> GHMLQNNTDYPFEANNPYMYHENPMEEGLSMLKLANLAEAALAFEAVCQAAPEREEAWRSLGLTQAENEKDGLAIIALNHARMLDPKDIAVHAALAVSHTNEHNANAALASLRAWLLSQPQYEQLGSVNLQADVDIDDLNVQSEDFFFAAPNEYRECRTLLHAALEMNPNDAQLHASLGVLYNLSNNYDSAAANLRRAVELRPDDAQLWNKLGATLANGNRPQEALDAYNRALDINPGYVRVMYNMAV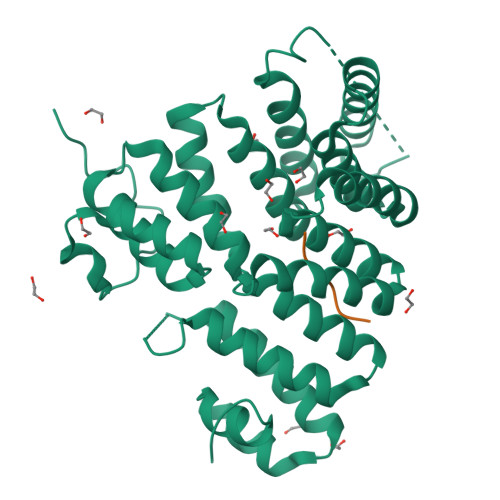SYSNMSQYDLAAKQLVRAIYMQVGGTTPTGEASREATRSMWDFFRMLLNVMNRPDLVELTYAQNVEPFAKEFGLQSMLL;> FNELSHL>[2x]GIDPFTMTPSEDFVVTDRGGIVENSHRVHAAVVDAKGRLLYALGNPTRMTLARSAAKPAQALAILETEGVAGYGFDDADIALMCASHSSEDRHIARTRAMLSKIKAEEADLRCGGHPSLSEMVNRSWIKQDFIPTAVCSNCSGKHVGM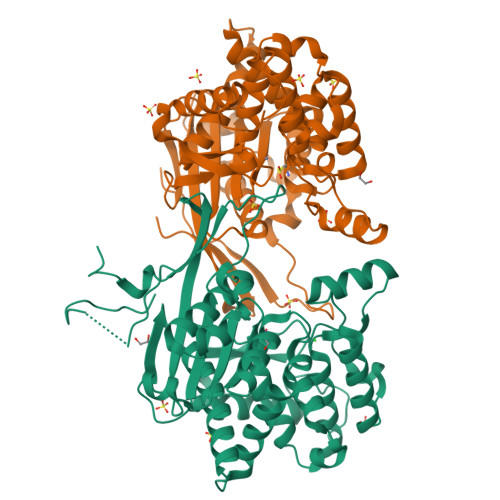LAGARAIGAGTDGYHLPDHPMQGRVKRTVAELCDLDAGDVEWGTDGCNLPTPAFPLDRLGRIYAKLASAADGSDAGEGQSTRCAALAHIFRAMARHPEMVAGEGRYCTMLMRAFDGALVGKLGADASYAIGVRASDATRQLGTDGALGISVKIEDGNLEMLYAVVTELLERLGIGSPDVRSQLASFHHPQRVNTMGVTTGGVSFPFKLRGSKSNVDDPRLAAVAR>MASGSMHLRPIATPYPVKEWLQPKRYKAHLMGTTYVYDFPELFRQASSSQWKNFSADVKLTDDFFISNELIEDENGELTEVEREPGANAIGMVAFKITVKTPEYPRGRQFVVVANDITFKIGSFGPQEDEFFNKVTEYARKRGIPRIYLAANSGARIGMAEEIVPLFQVAWNDAANPDKGFQYLYLTSEGMETLKKFDKENSV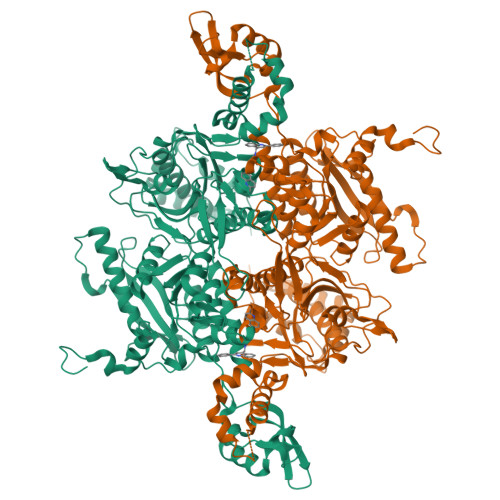LTERTVINGEERFVIKTIIGSEDGLGVECLRGSGLIAGATSRAYHDIFTITLVTCRSVGIGAYLVRLGQRAIQVEGQPIILTGAPAINKMLGREVYTSNLQLGGTQIMYNNGVSHLTAVDDLAGVEKIVEWMSYVPAKRNMPVPILETKDTWDRPVDFTPTNDETYDVRWMIEGRETESGFEYGLFDKGSFFETLSGWAKGVVVGRARLGGIPLGVIGVETRTVENLIPADPANPNSAETLIQEPGQVWHPNSAFKTAQAINDFNNGEQLPMMILANWRGFSGGQRDMFNEVLKYGSFIVDALVDYKQPIIIYIPPTGELRGGSWVVVDPTINADQMEMYADVNARAGVLEPQGMVGIKFRREKLLDTMNRLDDKYRELRSQLSNKSLAPEVHQQISKQLADRERELLPIYGQISLQFADLHDRSSRMVAKGVISKELEWTEARRFFFWRLRRRLNEEYLIKRLSHQVGEASRLEKIARIRSWYPASVDHEDDRQVATWIEENYKTLDDKLKGLKLESFAQDLAKKIRSDHDNAIDGLSEVIKMLSTDDKEKLLKTLKLEHHHHHH[3x]>[2x]MHHHHHHGENLYFQGSAPYASLTEIEHLVQSVCKSYRETCQLRLEDLLRQRSNIFSREEVTGYQRKSMWEMWERCAHHLTEAIQYVVEFAKRLSGFMELCQNDQIVLLKAGAMEVVLVRMCRAYNADNRTVFFEGKYGGMELFRALGCSELISSIFDFSHSLSALHFSEDEIALYTALVLINAHRPGLQEKRKVEQLQYNLELAFHHHLCKTHRQSILAKLPPKGKLRSLCSQHVERLQIFQHLHPIVV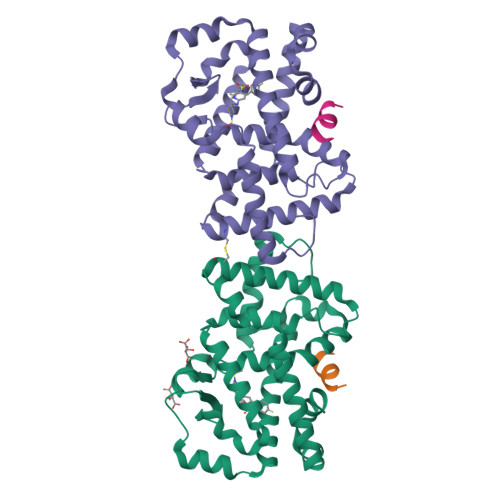QAAFPPLYKELFSGNS;>SLLKKLLD[2x]> MGDTAKPYFVKRTKDRGTMDDDDFRRGHPQQDYLIIDDHAKGHGSKMEKGLQKKKITPGNYGNTPRKGP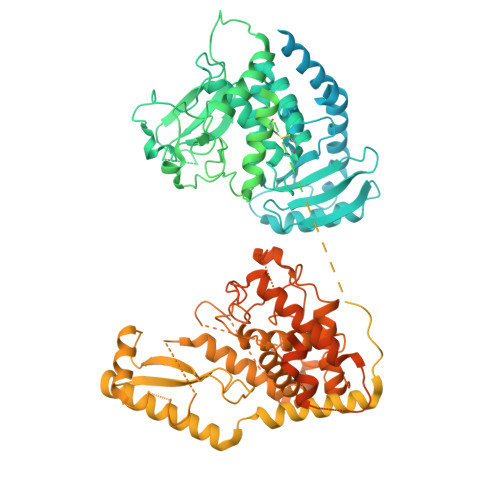CAVSSNPYAFKNPIYSQPAWMNDSHKDQSKRWLSDEHTGNSDNWREFKPGPRIPVINRQRKDSFQENEDGYRWQDTRGCRTVRRLFHKDLTSLETTSEMEAGSPENKKQRSRPRKPRKTRNEENEQDGDLEGPVIDESVLSTKELLGLQQAEERLKRDCIDRLKRRPRNYPTAKYTCRLCDVLIESIAFAHKHIKEKRHKKNIKEKQEEELLTTLPPPTPSQINAVGIAIDKVVQEFGLHNENLEQRLEIKRIMENVFQHKLPDCSLRLYGSSCSRLGFKNSDVNIDIQFPAIMSQPDVLLLVQECLKNSDSFIDVDADFHARVPVVVCREKQSGLLCKVSAGNENACLTTKHLTALGKLEPKLVPLVIAFRYWAKLCSIDRPEEGGLPPYVFALMAIFFLQQRKEPLLPVYLGSWIEGFSLSKLGNFNLQDIEKDVVIWEHTDSAAGDTGITKEEAPRETPIKRGQVSLILDVKHQPSVPVGQLWVELLRFYALEFNLADLVISIRVKELVSRELKDWPKKRIAIEDPYSVKRNVARTLNSQPVFEYILHCLRTTYKYFALPHKITKSSLLKPLNAITCISEHSKEVINHHPDVQTKDDKLKNSVLAQGPGATSSAANTCKVQPLTLKETAESFGSPPKEEMGNEHISVHPENSDCIQADVNSDDYKGDKVYHPETGRKNEKEKVGRKGKHLLTVDQKRGEHVVCGSTRNNESESTLDLEGFQNPTAKECEGLATLDNKADLDGESTEGTEELEDSLNHFTHSVQGQTSEMIPSDEEEEDDEEEEEEEEPRLTINQREDEDGMANEDELDNTYTGSGDEDALSEEDDELGEAAKYEDVKECGKHVERALLVELNKISLKEENVCEEKNSPVDQSDFFYEFSKLIFTKGKSPTVVCSLCKREGHLKKDCPEDFKRIQLEPLPPLTPKFLNILDQVCIQCYKDFSPTIIEDQAREHIRQNLESFIRQDFPGTKLSLFGSSKNGFGFKQSDLDVCMTINGLETAEGLDCVRTIEELARVLRKHSGLRNILPITTAKVPIVKFFHLRSGLEVDISLYNTLALHNTRLLSAYSAIDPRVKYLCYTMKVFTKMCDIGDASRGSLSSYAYTLMVLYFLQQRNPPVIPVLQEIYKGEKKPEIFVDGWNIYFFDQIDELPTYWSECGKNTESVGQLWLGLLRFYTEEFDFKEHVISIRRKSLLTTFKKQWTSKYIVIEDPFDLNHNLGAGLSRKMTNFIMKAFINGRRVFGIPVKGFPKDYPSKMEYFFDPDVLTEGELAPNDRCCRICGKIGHFMKDCPMRRKVRRRRDQEDALNQRYPENKEKRSKEDKEIHNKYTEREVSTKEDKPIQCTPQKAKPMRAAADLGREKILRPPVEKWKRQDDKDLREKRCFICGREGHIKKECPQFKGSSGSLSSKYMTQGKASAKRTQQES[(3R,4R)-4-hydroxy-1-{[5-(hydroxymethyl)pyridin-3-yl]methyl}pyrrolidin-3-yl]methyl dihydrogen 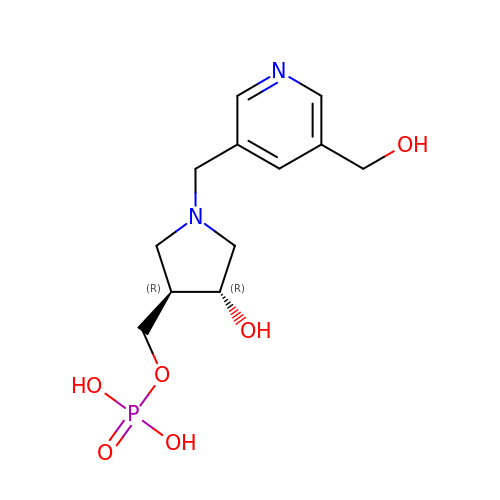phosphate | C12 H19 N2 O6 P | SZNYLPNTDKRZQR-NEPJUHHUSA-N>MATNGMRPIHPGEILRDEFLMEFDISPAALARALKVSAPTVNDIVREQRGISADMAIRLGRYFDTSAQFWMNLQS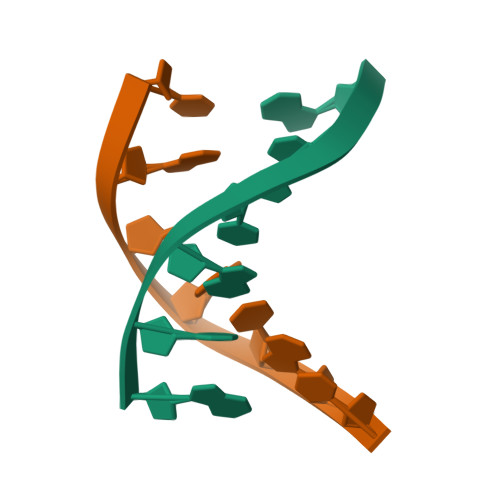EYSLATAYAANGKQIEHEIEPLLAHGGSHHHHHH[8x]>MSKTQEFRPLTLPPKLSLSDFNEFIQDIIRIVGSENVEVISSKDQIVDGSYMKPTHTHDPHHVMDQDYFLASAIVAPRNVADVQSIVGLANKFSFPLWPISIGRNSGYGGAAPRVSGSVVLDMGKNMNRVLEVNVEGAYCVVEPGVTYHDLHN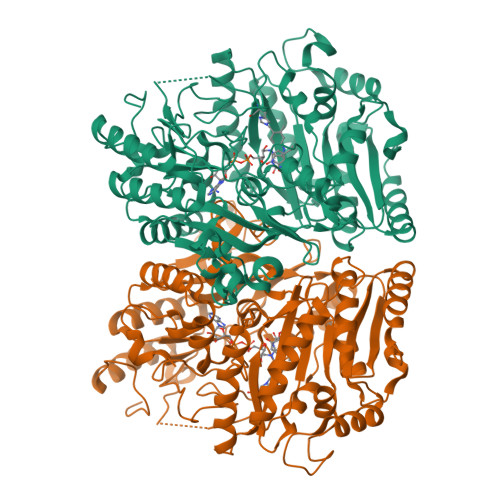YLEANNLRDKLWLDVPDLGGGSVLGNAVERGVGYTPYGDHWMMHSGMEVVLANGELLRTGMGALPDPKRPETMGLKPEDQPWSKIAHLFPYGFGPYIDGLFSQSNMGIVTKIGIWLMPNPRGYQSYLITLPKDGDLKQAVDIIRPLRLGMALQNVPTIRHILLDAAVLGDKRSYSSRTEPLSDEELDKIAKQLNLGRWNFYGALYGPEPIRRVLWETIKDAFSAIPGVKFYFPEDTPENSVLRVRDKTMQGIPTYDELKWIDWLPNGAHLFFSPIAKVSGEDAMMQYAVTKKRCQEAGLDFIGTFTVGMREMHHIVCIVFNKKDLIQKRKVQWLMRTLIDDCAANGWGGYRTHLAFMDQIMETYNWNNSSFLRFNEVLKNAVDPNGIIAPGKSGVWPSQYSHVTWKL[2x]>MLKTNIELKPKVEAFLNEEIKMFINGEFVSAIGGKTFETYNPATEDVLAVVCEAQEEDIDAAVKAARSAFESGPWAEMTTAERAHLIYKLADLIEEHREELAQLEALDNGKPYQVALDDDISATVENYRYYAGWTTKIIGQTIPISKDYLNYTRHEPVGVVGQIIPWNFPLVMSSWKMGAALATGCTIVLKPAEQTPLSLLYAAKLFKEAGFPNGVVNFVPGFGPEAGAAIVNHHDIDKVAFTGSTVTGKYIMRQSAEMIKHVTLELGGKSPNIILEDADLEEAINGAFQGIMYNHGQNCSAGSRVFVHRKHYETVVDALVKMANNVKLGAGMEKETEMGPLVSKKQQERVLNYIEQGKKEGATVAAGGERALEKGYFVKPT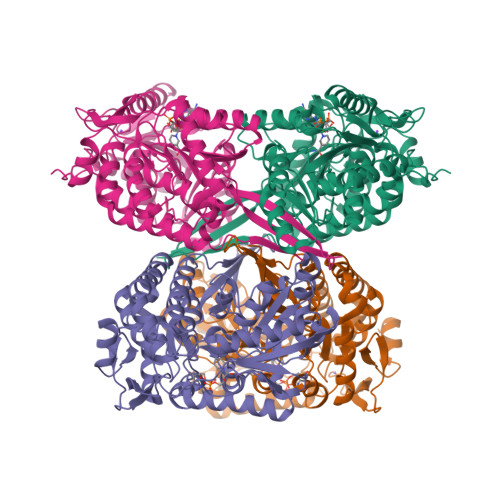VFTDVTDDMTIVKEEIFGPVVVVLPFDSTEEVIERANNSSYGLAAGVWTQNIKTGHQVANKLKAGTVWINDYNLENAAAPFGGYKQSGIGRELGSYALDNYTEVKSVWVNIK[4x]Here structural analysis of hydroxyketoacid aldolase from Sphingomonas wittichii RW1 (SwHKA) revealed a dynamic movement of the metal cofactor between two coordination spheres without protein scaffold rearrangements. Holo‐SwHKA forms a trimer of homodimers, in which each monomer adopts an (α/β)8 triosephosphate isomerase (TIM) barrel fold. In total, holo‐SwHKA contains six equivalent active sites; each of which is formed from amino acids from two different domain‐swapped dimers. The transition from M2+ R to M2+ A,S is induced by bidentate substrate binding and occurs without a concomitant rearrangement of the protein scaffold.

Notably, the formation of the overall hexameric assembly of apo‐SwHKA does not seem to require the presence of a metal cofactor. Crystals of WT apo‐SwHKA and mutant variants thereof were soaked with MgCl2 or MnCl2 to afford the holo‐enzyme. In the absence of metals, wild‐type apo‐SwHKA and apo‐S116A displayed similar melting temperatures (T m) of approximately 66 °C, while variant S116C showed a slightly lower stability of 62 °C, which suggests no substantial disruption of the protein fold.

> HHHNKVRTCWNEGRPALAGWLQLPGTLHAEALARLDYDAVVIDMQHSPIDFGQVAPMLIAIELGGAEPFVRTQVNDPSDIMKLLDAGAYGIIAPMVNTRAEAQTLASALHYSPRGLRSFGPRRPSLRYGSGYLAQASETVVGLAMIETREALANIDEILSVDGIDGVFIGPTDLALDLGHAPLVDTEEAEVVSAIAHVRERAHAAGKRVGIFCGSGGFARVKLAEGFDFVTAAPDLAMLSAAARQVIADARAL15,16-DIHYDROBILIVERDIN | 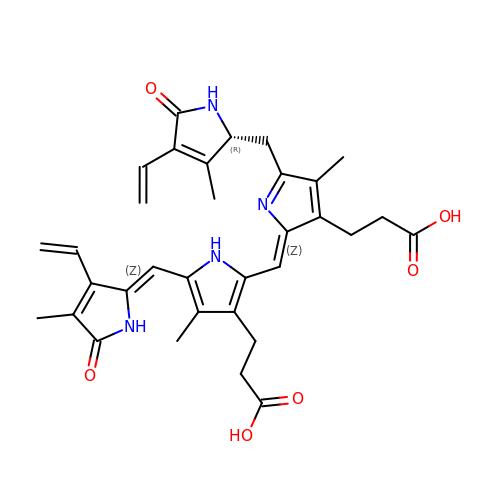C33 H36 N4 O6 | ZQHDSLZHMAUUQK-ZTYGKHTCSA-N>SNADSSRRQYQEKYKQVEQYMSFHKLPADFRQKIHDYYEHRYQGKMFDEDSILG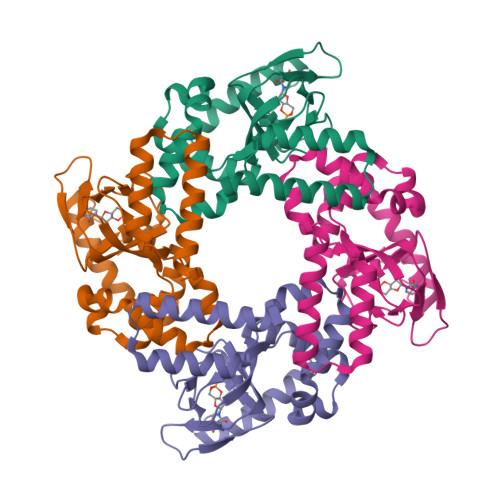ELNGPLREEIVNFNCRKLVASMPLFANADPNFVTAMLTKLKFEVFQPGDYIIREGTIGKKMYFIQHGVVSVLTKGNKEMKLSDGSYFGEICLLTRGRRTASVRADTYCRLYSLSVDNFNEVLEEYPMMRRAFETVAIDRLDRIGKKNSIL[2x]>[4x]HMVSLTERRKAETRMEIARAAARLFVGQGLRATRAED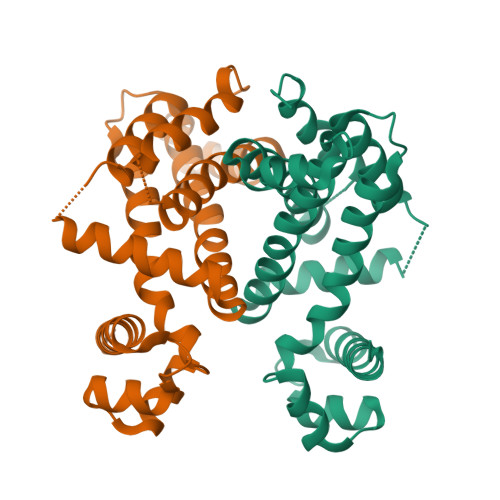IARAAGVAPRTFYRYFATKEEAVAPLYALGAERWVRAVREAPAELSPPEALERAVRHTLTPGAGVSAPSWEWARTLIRLAESSPALRKVWAEVCHSTERGLVQALAARMSGGDDNVAVRLAASPRLHFAAAVAGASVRVAAEHWASSSPQGARSPLEQALLNLEVLRGFAWEAGPAEEG>[3x]SNAMTDNPAVDKRDQILAAAEQLIAESGFQGLSMQ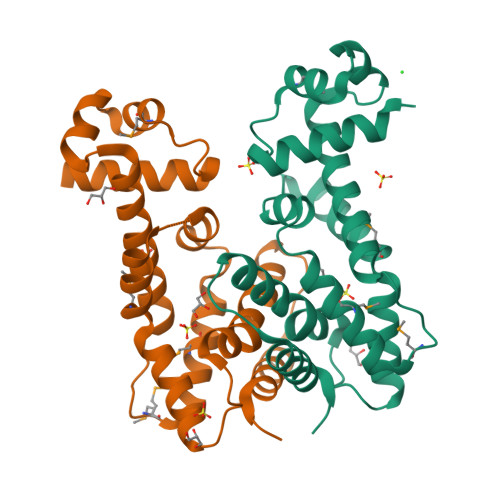KLANEAGVAAGTIYRYFSDKEHLLEEVRLNVAKRIASAVQAGVNDDMPLKERYRTMWLNIWNLAGSNLNAISNRVQYDSLPCTTRNKTWELERKMFAQVDRLFNQGKEEGVFKPLDNEVLSGLSFEASVALARKHALGFYQLDDDALEAAIEASWDAIIKH>[4x]HHHHHHFNLPPGNYKKPKLLYCSNGGHFLRILPDGTVDGTRDRSDQHIQLQLSAESVGEVYIKSTETGQYLCMDTDGLLYGSQTPNEECLFLERLEENHYNTYISKKHAEKNWFV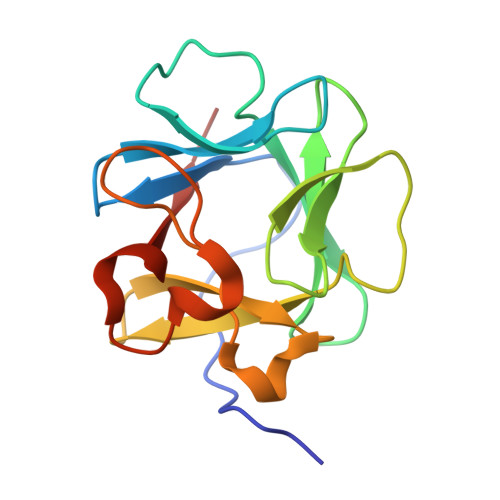GLKKNGSCKRGPRTHYGQKAILFLPLPVSSD7-O-phosphono-alpha-L-galacto-hept-2-ulopyranose 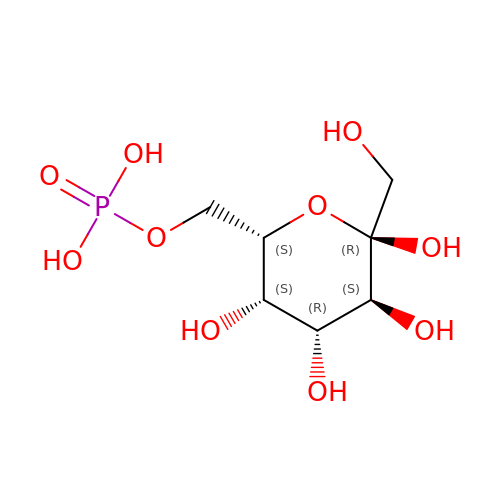| C7 H15 O10 P | CBIDVWSRUUODHL-CXNFULCWSA-N>ATSVVAWGGNNDWGEATVPAEAQSGVDAIAGGYFHGLALKGGKVLGWGANLNGQLTMPAATQSGVDAIAAGNYHSLALKDGEVIAWGGNEDGQTTVPAEARSGVDAIAAGAWASYALKDGKVIAWGDDSDGQTTVPAEAQSGVTALDGGVYTALAVKNGGVIAWGDNYFGQTTVPAEAQSGVDDVAGGIFHSLALKDGKVIAWGDNRYKQTTVPTEALSGVSAIASGEWYSLALKNGKVIAWGSSRTAPSSVQS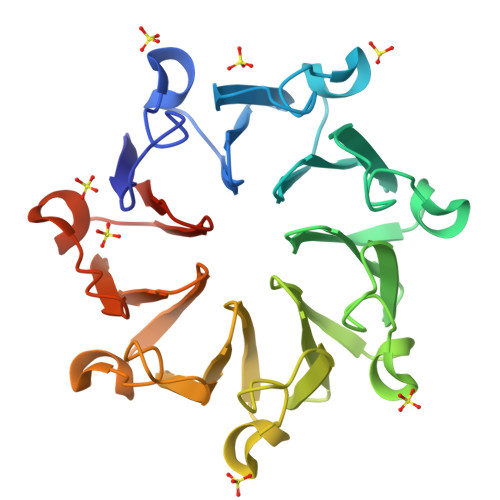GVSSIEAGPNAAYALKGGSGSGHHHHHH[6x]> ATFEIVNRCSYTVWAAASKGDAALDAGGRQLNSGESWTINVEPGTNGGKIWARTDCYFDD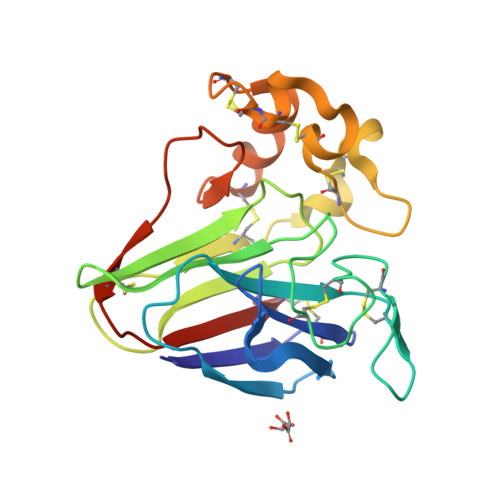SGSGICKTGDCGGLLRCKRFGRPPTTLAEFSLNQYGKDYIDISNIKGFNVPMDFSPTTRGCRGVRCAADIVGQCPAKLKAPGGGCNDACTVFQTSEYCCTTGKCGPTEYSRFFKRLCPDAFSYVLDKPTTVTCPGSSNYRVTFCPTA>[4x]MRSRRVDVM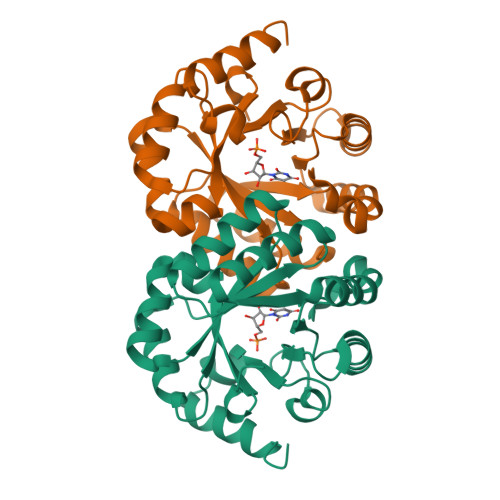DVMNRLILAMDLMNRDDALRVTGEVREYIDTVKIGYPLVLSEGMDIIAEFRKRFGCRIIADFKVADIPETNEKICRATFKAGADAIIVHGFPGADSVRACLNVAEEMGREVFLLTEMSHPGAEMFIQGAADEIARMGVDLGVKNYVGPSTRPERLSRLREIIGQDSFLISPGAGAQGGDPGETLRFADAAIAGRSIYLADNPAAAAAGIIESIKDLLNP Conjugative pili are widespread bacterial appendages that play important roles in horizontal gene transfer, in spread of antibiotic resistance genes, and as sites of phage attachment. The pilus is a polymer of the VirB2 protein (or pilin). The structures of the pED208 and F pilus are very similar, with overall dimensions of 87 Å in diameter and an internal lumen of 28 Å in diameter. Thus, selective binding of PG to pilins occurs in both F and pED208 pili, and thus, the F family of pili are polymers of a selective and stoichiometric protein-PG complex unit.

During the process of helical reconstruction, as the resolution was increased, an additional separate density became clearly visible and readily interpretable as a phospholipid. For the F pilus, it became apparent during the process of helical reconstruction that two populations of filaments were present, differing slightly in the rise between subunits (see below). Instead, two 5.0 Å resolution electron density maps were generated for the two F pilus populations. For pED208, the angle between adjacent subunits is 28.2° and the rise is 12.1 Å, while for the two F pilus structures, the helical parameters were 27.9° with a rise of 13.2 Å and 28.1° with a rise of 12.5 Å, respectively. Superposition of the structures of pED208 and F TraA reveals very similar overall structures (root-mean-squared deviation in Cα positions between pED208 and F [13.2 Å rise] of 1.4 Å and between pED208 and F [12.5 Å rise] of 1.5 Å) with slightly different boundaries for secondary structures. Also, the TraA pilin structures in the two F pilus forms are virtually identical (root-mean-squared deviation in Cα positions of 0.7 Å). Thus, with the structures and helical parameters of the two F pilus forms being so similar, functional differences between them are unlikely to arise but cannot be excluded. The amino acid sequences of both the orthologous pED208 and F pilus TraA pilin are similar, except for the F pilin N terminus, which is 4 amino acids (aa) longer. This longer N terminus could not be traced in the F pilus density maps and thus must be disordered. Indeed, the presence of phospholipid in the F pilus was also confirmed by MS; however, this time a PG species, PG 33:1 (16:0, ΔC17:0), was the major phospholipid observed in the F pilus after PLA2 treatment.

>[75x]QDLMASGNTTVKATFGKDSSVVKWVVLAEVLVGAVMYMMTKNVKFLAGFAIISVFIAVGMAVVGL4-methyl-3-{[6-(methylsulfonyl)quinolin-4-yl]amino}phenol 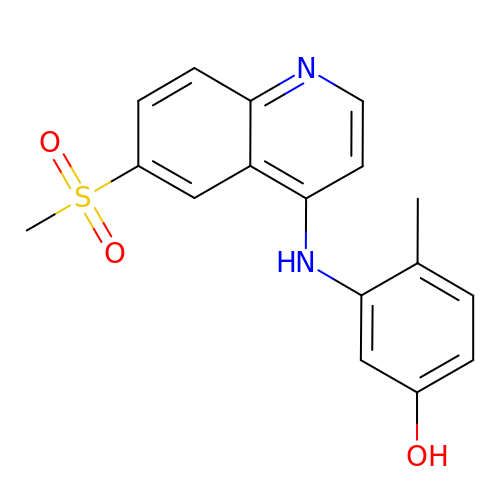| C17 H16 N2 O3 S | BVHZLDLRNBQWRF-UHFFFAOYSA-N(1R,2R)-3-[(S)-amino(carboxy)methyl]cyclopropane-1,2-dicarboxylic acid | 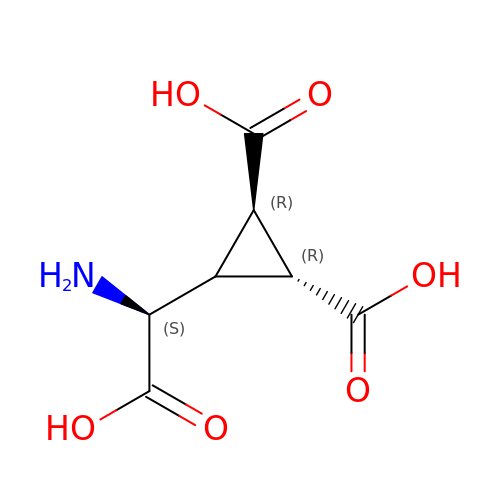C7 H9 N O6 | MATPZHBYOVDBLI-JJYYJPOSSA-N> SIVTKSIVNADAEARYLSPGELDRIKSFVLSGARRVRIAQTLTENRERIVKQAG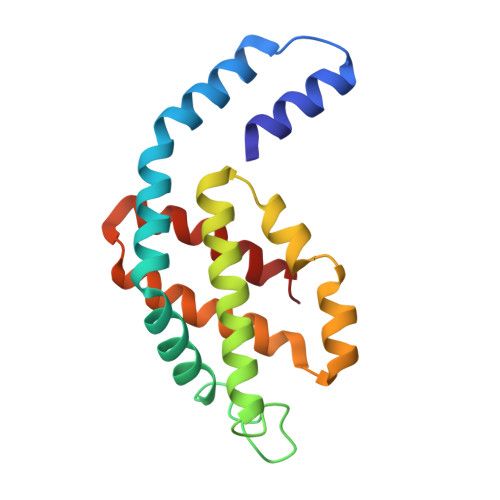DQLFQKRPDVVSPGGNAYGEEMTATCLRDLDYYLRLVTYGIVSGDVTPIEEIGLVGVREMYKSLGTPISAVAEGVKCMKSVASSLLSGEDSAEAGFYFDYVVGAMQ> ACYXPDYLCADEY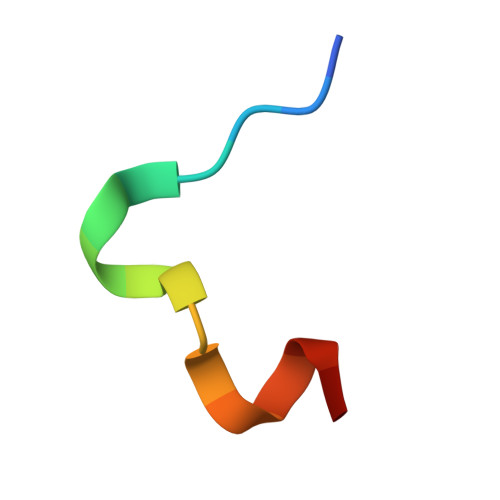CAX2-(2-HYDROXY-PHENYL)-1H-INDOLE-5-CARBOXAMIDINE 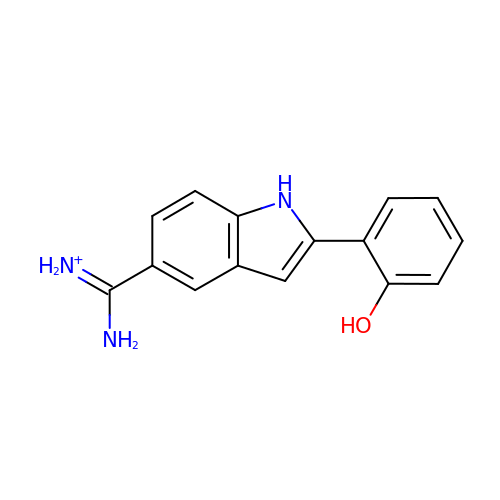| C15 H14 N3 O | JPGNPKIYCTXJPG-UHFFFAOYSA-O ETHACRYNIC 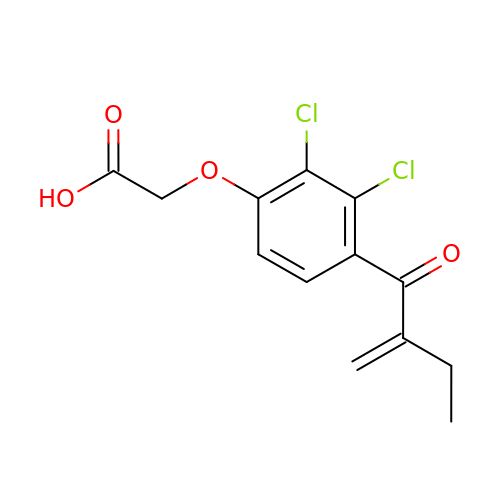ACID | C13 H12 Cl2 O4 | AVOLMBLBETYQHX-UHFFFAOYSA-N>MASMGTLAF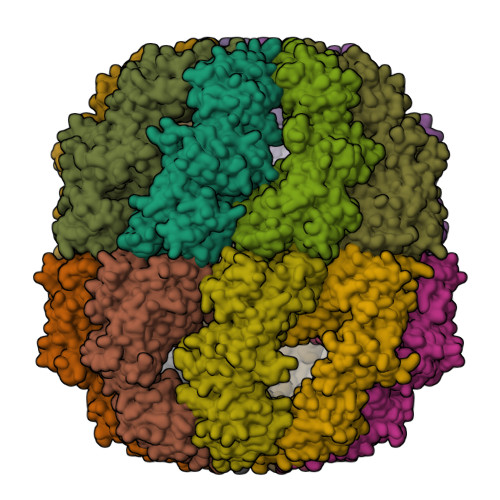DEYGRPFLIIKDQDRKSRLMGLEALKSHIMAAKAVANTMRTSLGPNGLDKMMVDKDGDVTVTNDGATILSMMDVDHQIAKLMVELSKSQDDEIGDGTTGVVVLAGALLEEAEQLLDRGIHPIRIADGYEQAARVAIEHLDKISDSVLVDIKDTEPLIQTAKTTLGSKVVNSCHRQMAEIAVNAVLTVADMERRDVDFELIKVEGKVGGRLEDTKLIKGVIVDKDFSHPQMPKKVEDAKIAILTCPFEPPKPKTKHKLDVTSVEDYKALQKYEKEKFEEMIQQIKETGANLAICQWGFDDEANHLLLQNNLPAVRWVGGPEIELIAIATGGRIVPRFSELTAEKLGFAGLVQEISFGTTKDKMLVIEQCKNSRAVTIFIRGGNKMIIEEAKRSLHDALCVIRNLIRDNRVVYGGGAAEISCALAVSQEADKCPTLEQYAMRAFADALEVIPMALSENSGMNPIQTMTEVRARQVKEMNPALGIDCLHKGTNDMKQQHVIETLIGKKQQISLATQMVRMILKIDDIRKPGESEE[4x]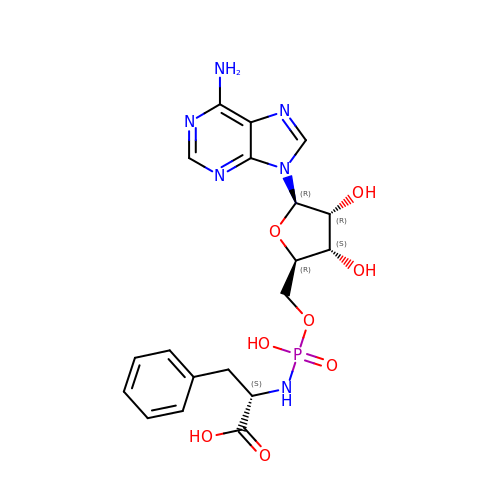(2~{S})-2-[[[(2~{R},3~{S},4~{R},5~{R})-5-(6-aminopurin-9-yl)-3,4-bis(oxidanyl)oxolan-2-yl]methoxy-oxidanyl-phosphoryl]amino]-3-phenyl-propanoic acid | C19 H23 N6 O8 P | OXCQKAQOLIIWJO-URQYDQELSA-N> EVDKRREINNEHPLLMMPLYANGEEFNQGKYTFWGGDTLTGKWENIPDDLKPYTVIQLHPDDLPKRDGAARDFYEHMLEEAAKYVNPKTGKNEPIPVILTVYTAGNMPYYTSAHWLSTSWIDKMYQKYPNLHGIFSTESYWIWANDIENKAADYLKVSAKNGGYFIWAEQNSGSAIEKAFGKNGKIAFQKSVDKYWKNLIFMFKNTPAAEGNDSTTESYMKGLWLSNHTYQWGGLMDTWKWYETGKWKLFASGNIGKSQGDRQWLTEPESMLGEEALGVYLNGGVVYNFEHPAYTYGVNNKESLLFSEVIKEFFRYVIAHPAPSKEKVLEDTKVFIHGDYSNKGNGKFFVNVNTDREQTPLYMTGRYNVIPAIPGVLKTDKLKESVSSSRIQIKEITSPEFSSTQARKEYLNKLYPMNYEGDIFAQKLDNRWFVYNYKVNENVKQTGKLKFNSLEMNVEFEPHTYGIFERISNGLKVNLNNFRTNKDSLWSNAQDANQAKKLPQLTKKGAIKWIEEHYIKDTQFGEKRVTKIVLRGIDKLPTIHSLSGTNNSYDQPSLNFDQKNHMVTITINSNGNLEFELHFLE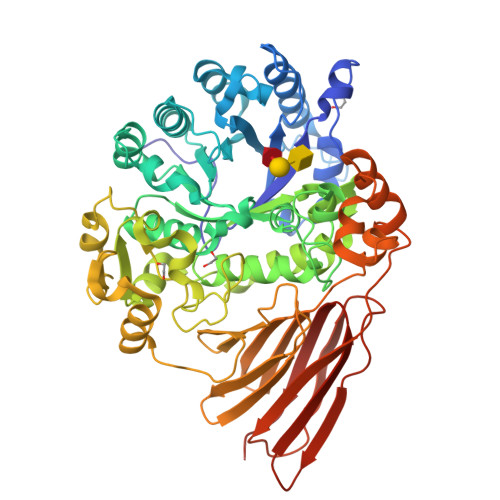HTRAPPPPPLRSGC>GPLGSPQMAQGTLIRVTPEQPTHAVCVLGTLTQLDICSSAPDDCTSFSINASPGVVVDIAHSPPAKKKSTGSSTWPLDPGVEVTLTMKAASGSTGDQKVQISYYGPKTPPVKALLYLTAVEISLCADITRTGKVKPTRAVKDQRTWTWGPCGQGAILLVNCDRDNLESSAMDCEDDEVLDSEDLQDMSLMTLSTKTPKDFFTNHTLVLHVARSEMDKVRVFQATRGKLSSKCSVVLGPKWPSHYLMVPGGKHNMDFYVEALAFPDTDFPGLITLTISLLDTSNLELPEAVVFQDSVVFRVAPWIMTPNTQPPQEVYACSIFENEDFLKSVTTLAMKAKCKLTICPEEENMDDQWMQDEMEIGYIQAPHKTLPVVFDSPRNRGLKEFPIKRVMGPDFGYVTRGPQTGGISGLDSFGNLEVSPPVTVRGKEYPLGRILFGDSCYPSNDSRQMHQALQDFLSAQQVQAPVKLYSDWLSVGHVDEFLSFVPAPDRKGFRLLLASPRSCYKLFQEQQNEGHGEALLFEGIKKKKQQKIKNILSNKTLREHNSFVERCIDWNRELLKRELGLAESDIIDIPQLFKLKEFSKAEAFFPNMVNMLVLGKHLGIPKPFGPVINGRCCLEEKVCSLLEPLGLQCTFINDFFTYHIRHGEVHCGTNVRRKPFSFKWWNMVP[2x];>XYRDHHYRHPKYC[2x]

The peptidylarginine deiminase enzymes (PADIs, or PADs, herein referred to as PADIs) catalyse the post-translational conversion of protein arginine residues to non-coded citrulline, in a process termed citrullination or peptidylarginine deimination. PADI4 possesses a nuclear localisation sequence and targets a variety of nuclear substrates, including core and linker histones, through which it modulates gene expression and chromatin compaction. PADIs require calcium for catalysis, and the sequential binding of calcium ions results in a large structural rearrangement that forms the active site cleft. We report PADI4_3, a cell-active inhibitor specific for the active conformation of PADI4; PADI4_7, an inert binder, which we functionalise for the isolation and study of cellular PADI4; and PADI4_11, a cell-active PADI4 activator.

The lead inhibitory peptide, PADI4_3, binds the active form of PADI4 and inhibits activity both in vitro and in cells, with higher potency and isozyme selectivity than previous compounds. We determined the structure of PADI4_3-bound PADI4 by cryoEM to an overall resolution of 3.1 Å. Additionally, well-defined density for the whole cyclic peptide was observed in both monomers, allowing us to assign all residues unambiguously. Unusually for peptides derived from RaPID selections, PADI4_3 itself does not adopt any secondary structure elements and relatively few intramolecular hydrogen bonds are observed within PADI4_348. The structure confirmed that PADI4_3 is a substrate-competitive inhibitor that binds within the active site of PADI4. Although PADI4_3 occupies the substrate binding site, rather than directly mimicking substrate binding by directing an arginine towards the active site, a histidine residue, H4, occupies this position. 760 Å2 of surface area is buried (per monomer) and, in line with its nanomolar binding affinity, there are many specific intermolecular interactions between PADI4 and PADI4_3 across this interface. This includes a bifurcated hydrogen bond between PADI4 R374 and the carbonyls of the PADI4_3 D3 backbone and the N-terminal acetyl group. Hydrogen bonds between the side chains of PADI4_3 R2 and PADI4 D344, PADI4_3 D3 and PADI4 H640, PADI4_3 H4 and PADI4 D350, and PADI4_3 H5 and PADI4 S468 are also observed. In line with the selectivity observed in COLDER assays, many of these residues are not conserved in other PADI isozymes or mouse PADI4. This is most pronounced for H640, which is not conserved in PADI1, PADI2 or mPADI4, and D344, which is not conserved in any of the other human PADIs.> ALRPKLSEEQQRIIAILLDAHHKTYDPTYSDFCQFRPPVRVNDGGGSVTLELSQLSMLPHLADLVSYSIQKVIGFAKMIPGFRDLTSEDQIVLLKSSAIEVIMLRSNESFTMDDMSWTCGNQDYKYRVSDVTKAGHSLELIEPLIKFQVGLKKLNLHEEEHVLLMAICI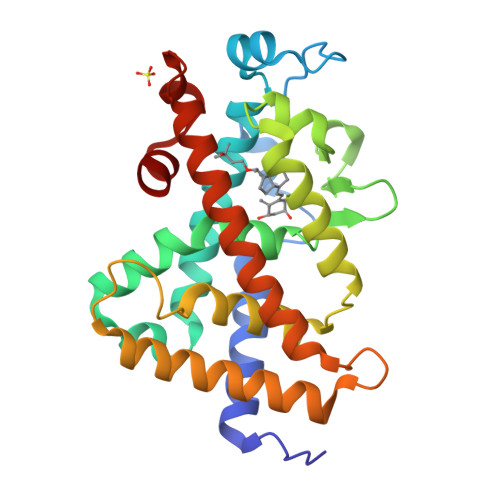VSPDRPGVQDAALIEAIQDRLSNTLQTYIRCRHPPPGSHLLYAKMIQKLADLRSLNEEHSKQYRCLSFQPECSMKLTPLVLEVFG> MKLDIKKTFSNRSDRVKGIDFHPTEPWVLT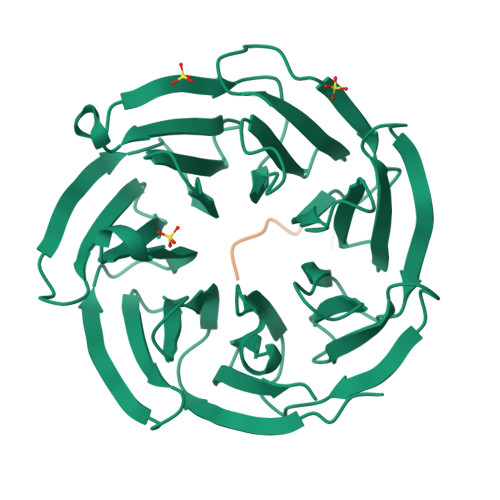TLYSGRVELWNYETQVEVRSIQVTETPVRAGKFIARKNWIIVGSDDFRIRVFNYNTGEKVVDFEAHPDYIRSIAVHPTKPYVLSGSDDLTVKLWNWENNWALEQTFEGHEHFVMCVAFNPKDPSTFASGCLDRTVKVWSLGQSTPNFTLTTGQERGVNYVDYYPLPDKPYMITASDDLTIKIWDYQTKSCVATLEGHMSNVSFAVFHPTLPIIISGSEDGTLKIWNSSTYKVEKTLNVGLERSWCIATHPTGRKNYIASGFDNGFTVLSLGNDE;> CTFKTKTN>[6x]GSREEYPDIDSEVRAILLSHAQNGITISSIKSEYRKLTGNPFPLHD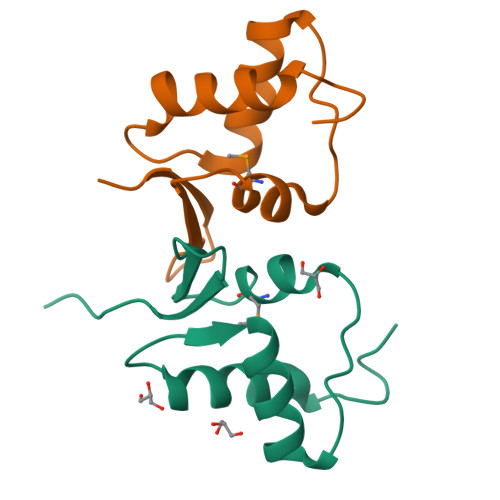NVTDFMLTIPNVTAECSESGKRIFNLKASLK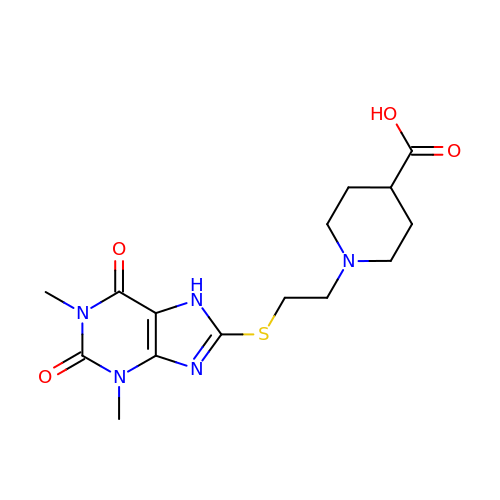1-{2-[(1,3-dimethyl-2,6-dioxo-2,3,6,7-tetrahydro-1H-purin-8-yl)sulfanyl]ethyl}piperidine-4-carboxylic acid | C15 H21 N5 O4 S | SRBZGKUKUDZIDS-UHFFFAOYSA-N>[2x]MNKYSQFLIFAAVLVSACNSPKTTKEMKSTDDCPEKVTFTPEQIDHLGITDTNHLSAASKRALKWPTDLGNEWFIQFGPLQPLKGDLAYEEGVVRRDPSAIIKENGKYYVWYSKSTGPTQGFGGDIEKDKVFPWDRCDIWYATSEDGWTWKEEGPAV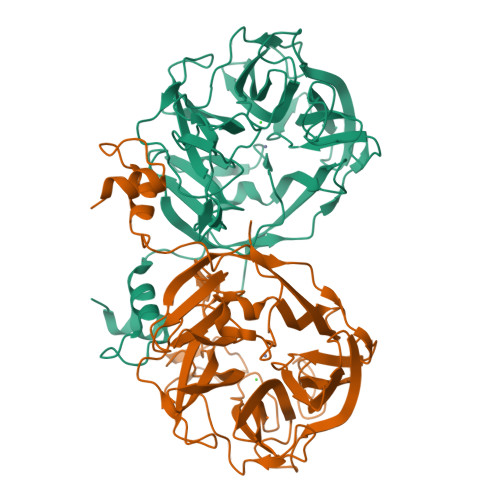TRGEKGAYDDRSVFTVEIMKWEDKYYLCYQTVKSPYNVRVKNQVGLAWADSPDGPWTKSEEPILSPADNGVWKGEEQDRFAVIKKGDFDSHKVHDPCIIPYKGKFYLYYKGEQMGEAITFGGRQIRHGVAIADNPKGPYVKSPYNPISNSGHEICVWPYNGGIASLITTDGPEKNTIQWAPDGINFEIKSVIPGVNAHAIGLNRTADVEKEPTEILRWGLTHIYNNGDYQSIMRFSSERKTRHVAKGVKKQ>GSSHHHHHHSSGLVPRGSHMRTAPPGSAGQPPDAAVTGLHVQGGRLLEGNGNDFVMRGVNHAHTWYPGQTRSLA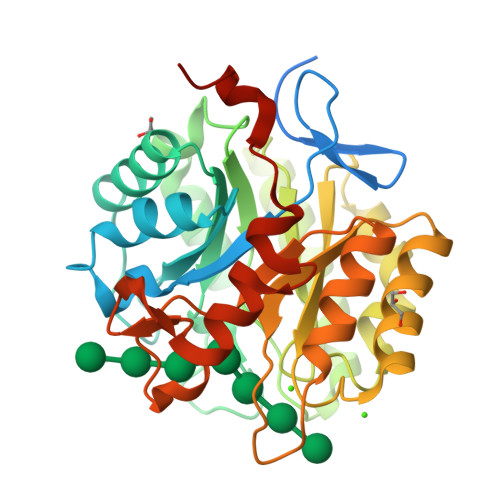DIKALGANTVRVVLSDGHRWTRNGPADVAAVIDRCKANRLICVLEVHDTTGYGEEPAAGTLDHAADYWISLMDVLAGQEDYVIVNIGNEPWGNTDPAGWTAPTIAAVKKLRAAGLAHTLMIDAPNWGQDWQGVMRADARSVYEADPTGNLLFSIHMYSVFDTAAEIDDYLEAFVDAGLPLVIGAFGGPPDQWGDPDEDTMLAAAERLRLGYLAWSWSGNTDPVLDLAIGFDPDRLSGWGQRVFHGVHGIGETSREATVFGKLAALEHHHHHH[2x]7-propyl-3-[2-(pyridin-3-yl)-1,3-thiazol-5-yl]-1,7-dihydro-6H-pyrazolo[3,4-b]pyridin-6-one 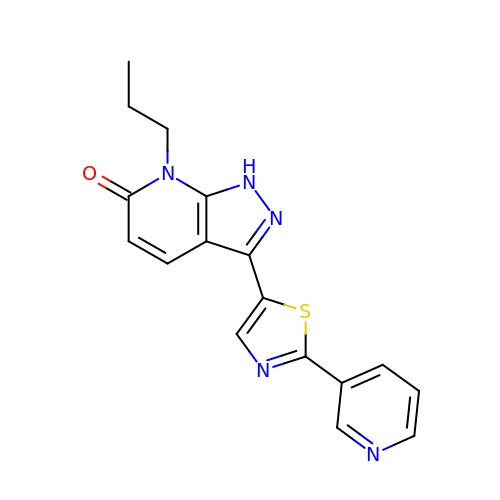| C17 H15 N5 O S | VOOCDNWLHBWIJZ-UHFFFAOYSA-N>MKQLTILGSTGSIGCSTLDVVRHNPEHFRVVALVAGKNVTRMVEQCLEFSPRYAVMDDEASAKLLKTMLQQQGSRTEVLSGQQAACDMAALEDVDQVMAAIVGAAGLLPTLAAIRAGKTILLANKESLVTCGRLFMDAVKQSKAQLLPVDSEHNAIFQSLPQPIQHNLGYADLEQNGVVSILLTGSGGPFRETPLRDLATMTPDQACRHPNWSMGRKISVDSATMMNKGLEYIEARWLFNASASQMEVLIHPQSVIHSMVRYQDGSVLAQLGEPDMRTPIAHTMAWPNRVNSGVKPLDFCKLSALTF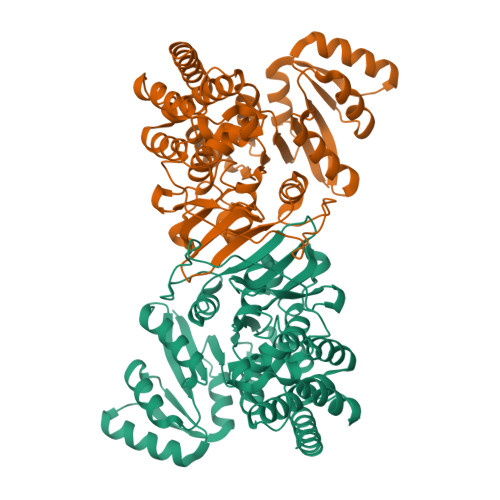AAPDYDRYPCLKLAMEAFEQGQAATTALNAANEITVAAFLAQQIRFTDIAALNLSVLEKMDMREPQCVDDVLSVDANAREVARKEVMRLAS[2x]> GSHMSGEDAEVRAVSEDVSNGSSGSPSPGDTLPWNLGKTQRSRRSGGGAGSNGSVLDPAERAVIRIADERDRVQKKTFTKWVNKHLIKAQRHISDLYEDLRDGHNLISLLEVLSGDSLPREKGRMRFHKLQNVQIALDYLRHRQVKLVNIRNDDIADGNPKLTLGLIWTIILHFQISDIQVSGQSEDMTAKEKLLLWSQRM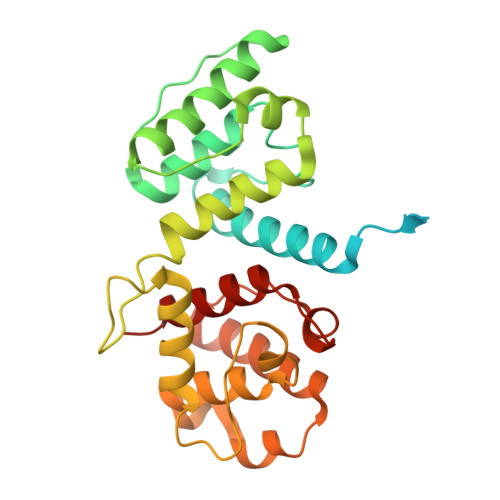VEGYQGLRCDNFTSSWRDGRLFNAIIHRHKPLLIDMNKVYRQTNLENLDQAFSVAERDLGVTRLLDPEDVDVPQPDEKSIITYVSSLYDAMPRVP> MSKAKIGIVTVSDRASAGITADISGKAIILALNLYLTSEWEPIYQVIPDEQKVIETTLVKMADIQDCCLIVTTGGTGPAKRDVTPEATEAVCDRMMPGFGELMRAESLKEV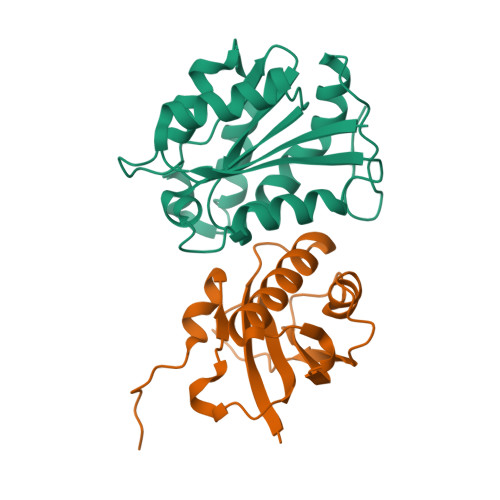PTAILSRQTAGLRGDSLIVNLPGDPASISDCLLAVFPAIPYCIDLMEGPYLECNEAMIKPFRPKAKLEHHHHHH;> MVRGIRGAITVNSDTPTSIIIATILLLEKMLEANGIQSYEELAAVIFTVTEDLTSAFPAEAARQIGMHRVPLLSAREVPVPGSLPRVIRVLALWNTDTPQDRVRHVYLSEAVRLRPDLESAQLEHHHHHH>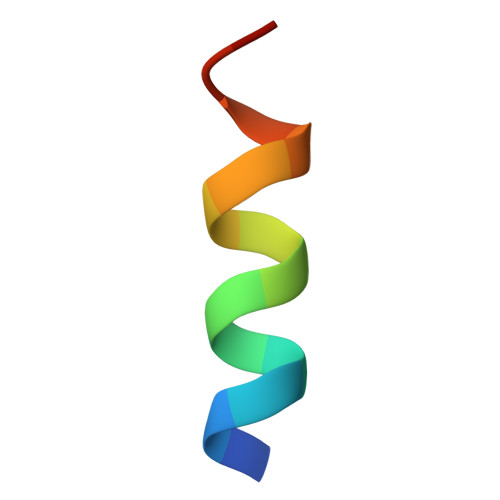 GVVKQKLAEVILKKQ The main protease (Mpro) of the betacoronavirus SARS-CoV-2 is an attractive target for the development of treatments for COVID-19. Starting from crystal structures of the Mpro in complexes with the Hepatitis C virus NS3/4A protease inhibitors boceprevir and telaprevir, we optimized the potency of the alpha-ketoamide boceprevir against the Mpro by replacing its P1 cyclobutyl moiety by a γ-lactam as a glutamine surrogate. In line with our original goal of identifying broad-spectrum inhibitors that target the main protease of coronaviruses and the 3C protease of enteroviruses, we also assessed the inhibitory potency of MG-78 against the Mpro of the alphacoronavirus HCoV NL63 and the 3Cpros of enterovirus A71 (EV-A71) and Coxsackievirus B3 (CVB3). Finally, coronavirus Mpros feature a catalytic dyad comprising a Cys…His pair, whereas enterovirus 3Cpros have a catalytic triad consisting of Cys…His…Glu(Asp).

Using 10 µM Dabcyl-KEALFQ↓GPPQFE(-Edans)-NH2 (↓ indicates the cleavage site) as a FRET substrate, we found IC50 values for MG-78 of 6.7 ± 2.2 μM against the EV-A71 3Cpro and 1.45 ± 0.40 μM against CVB3 3Cpro. Crystals of the EV-A71 3Cpro complex with MG-78 were grown in cubic space group P432 and yielded useful diffraction data extending to a Bragg spacing of 2.07 Å, whereas the CVB3 3Cpro complex gave crystals in space group C2 that diffracted to 1.65 Å. Compound MG-78 binds along the substrate-binding cleft in both proteases. Similar to the situation in the coronavirus Mpro, the nucleophilic attack of the catalytic residue (here Cys147) onto the α-keto group of the α-ketoamide warhead leads to the formation of a thiohemiketal, with a covalent bond between the sulfur of the catalytic Cys and the α-carbon. The carbonyl of the γ-lactam accepts hydrogen bonds from His161 Nε2 and the side-chain hydroxyl of Thr142. In the EV-A71 3Cpro structure, the gem-dimethyl groups of the cyclopropyl proline make contacts with the side-chains of Leu127 and Ser128 of the “beta-ribbon” of the protease. In particular the latter interaction, with a distance of 3.3 Å between one of the methyl groups and the Oγ of Ser128, has to be considered energetically unfavorable and may well constitute one of the reasons for the limited inhibitory potency of compound MG-78. The same could be true for the short distance (3.3 Å) between the Cγ atom of the proline and the same Ser128 side-chain. In the EV-A71 3Cpro structure, but not in the CVB3 structure, the P3 tert-butyl side-chain makes contacts to the ligand in a neighboring protease molecule in the crystal lattice. Whereas the crystal structure of MG-78 in complex with the SARS-CoV-2 Mpro revealed an ideal fit, those of the complexes with CVB3 3Cpro and EV-A71 3Cpro demonstrated some steric incompatibilities that likely reduce the inhibitory potency.

> PSLDFALSLLRRNIRQVQTDQGHFTMLGVRDHLAVLPRHSQPGKTIWVEHKLVRIVDAVELVDEQGVNLELTLVTLDTNEKFRDITRFIPETISPASDATLVINTEHMPSMFVPVGDVVQYGFLNLSGKPTHRTMMYNFPTKAGQCGGVVTAVGKVIGIHIGGNGRQGFCAALKRGYFCSEQ(4~{a}~{S},8~{a}~{R})-2-cycloheptyl-4-[4-(2-hydroxyethyloxy)-3-[2-(2-oxidanylideneimidazolidin-1-yl)ethoxy]phenyl]-4~{a},5,8,8~{a}-tetrahydrophthalazin-1-one 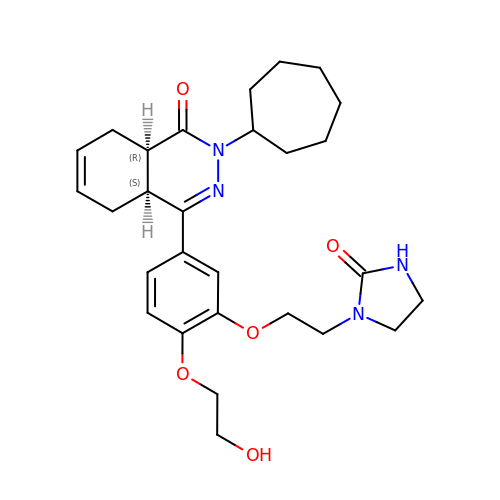| C28 H38 N4 O5 | NSRKPNKUYKBHPD-XZOQPEGZSA-N> MVMRRCSYNVHPTWYMMPLRAYHMPGWKTKVSTKDVRTREQREADRKVRQIEKLPRPQALHDFQYPYEKTVLSDTMFQYPVYENELDTPHLFNITEPPDFFVYWNVSDFERTSYPPLPEEDHRLLLPLSGSAPWKQHRKRSLKYLRKHEILPNYLPHVRQDVNLSVVFPGVYATRARLCEETGEPLPPPPPVSRMTHRNFWMTAHCGNYIELADLQHPPSIFFLDTVSATGQGKAVEKDATEEGSDEVWYTLIIASPDYPFRVPASVDASTQRGFFLNYMMSNLKGGGNSTVLEEYESEQRQNNQKRQHLEELVRNPAPIAKEGDVIVSYTPPLPTEDAGTTRHICMLFKQRSYVSGASCALDDSKASFAARANFRLHAQHRDGIPSSSVEMLSRIEQV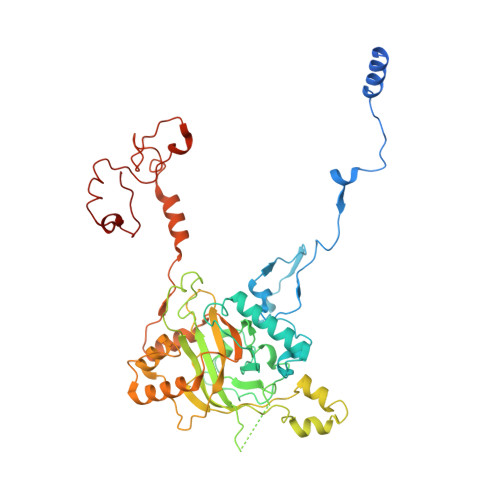LPPDPSAVTFFQTKWDIQVQEFYESRGMLEPAAPLDEEIEAILAYHARKPSELRVRARHRPDGSTNVGDDPNFWAQAEPTRMMDGSMLSLWSRRTTLGANGVPITYRR1,7-di-O-phosphono-D-glycero-beta-D-manno-heptopyranose 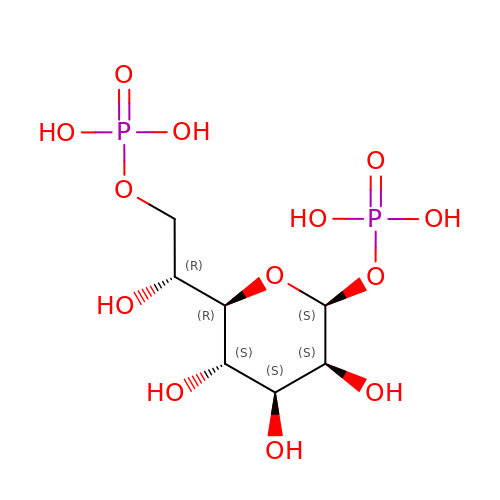| C7 H16 O13 P2 | LMTGTTLGDUACSJ-QTNLNCNHSA-N> AQVINTFDGVADYLQTYHKLPDNYITKSEAQALGWVASKGNLADVAPGKSIGGDIFSNREGKLPG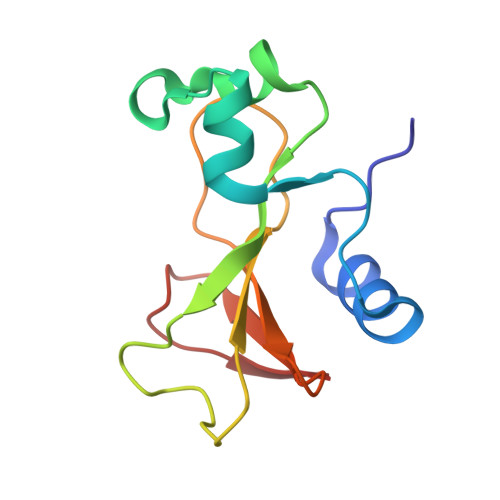KSGRTWREADINYTSGFRNSDRILYSSDWLIYKTTDHYQTFTKIR> MALPLDFTNSDVVMGALTKAVGRLCLDVTGYDVVEADETIPKPEGPYILVDLSLLTPLDWATNEVVDEDGVVHTAHNYTASYTLTAYRGKPHWALSRVHQAFGLPFLREKYFPTGSPYAYSSTSNIARMRVPLNQQMFENRARTIVTFNATFVEKDLGTFEDIEHIIIGIDVDNPSGP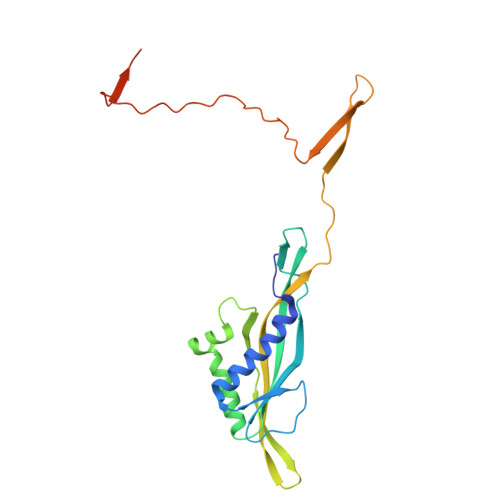PIGIGADYDKGVKPGGDDPGLPPKPNPPIVYHDAIAQVCMATPVIDKPALISDKTGE> SNAMDFIIVDDSVFDLFTQEKLLLKSGLTTSVRTFNSAQAAIDHLRSQGADIPDTVILLDLQMPGINGFEFTEHYGMLPEAVRARIRLFMI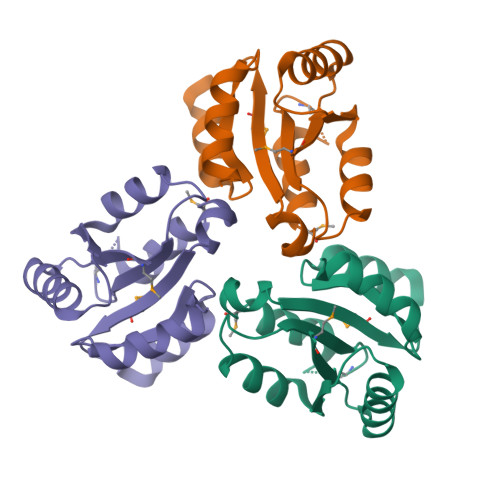SSTVDISDIEQAEANPHIIQLLPKPLEIPLLRELLKRWFPSI> MLSCKGVLLMRHIGQDVPRRHTHFVLESRLMYE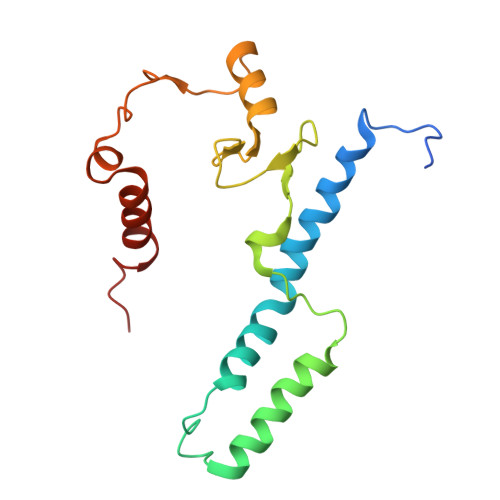KSFRDEWLRSLCQGLANVDEPLAKSLSGLPQQMLQRKVTCFSYNQFGLFKVPYYRLANVDRYYAVQGALGTREWVPYANVSSWTMNKMVRSGNILVHRVHYKGWGTDNALNQGGWEHRWNKVMQRNALQYNRI>[4x]NEKFRPEMLQGKKVIVTGASKGIGREIAYHLAKMGAHVVVTARSKEALQKVVARCLELGAASAHYIAGSMEDMTFAEEFVAEAGNLMGGLDMLILNHVLYNRLTFFHGEID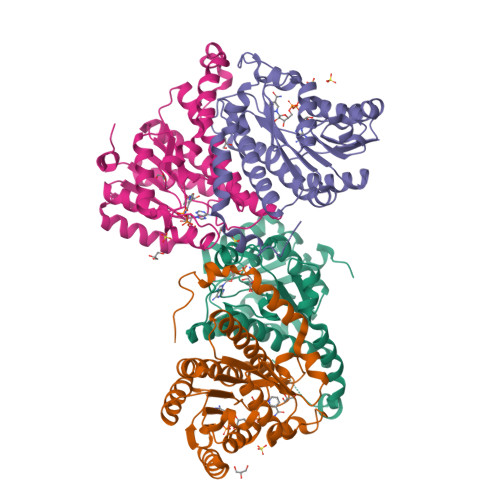NVRKSMEVNFHSFVVLSVAAMPMLMQSQGSIAVVSSVAGKITYPLIAPYSASKFALDGFFSTLRSEFLVNKVNVSITLCILGLIDTETAIKATSGIYLGPASPKEECALEIIKGTALRQDEMYYVGSRWVPYLLGNPGRKIMEELSAAEYNWDNVLSNEKLYGRW> AKCVSYGVAQIKAPALHSQGYTGSNVKVAVLASGIDSSHPDLNVAGGASFVPSETNPFQDNNSHGTHVAGTVLAVAPSASLYAVKVLGADGSGQASWIINGIEWAIANNMDVINMSLGSPSGSAALKAAVDKAVASGVVVVAAAGNSGTSGSSSTVSYPAKYPSVIAVGAVDSSNQRAPFSSVGPELDVMAPGVSICSTLPGGKYGALSGTAMASPHVAGAAALILSKHPNWTNTQVRSSLENTA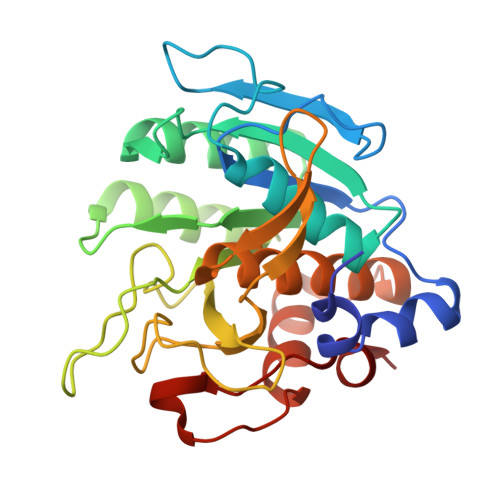TKLGDSFYYGKGLINVEAAAQ>GSCKLPVKKATVVYQGERVKIQEKFKNGMLHGDKVSFFCKNKEKKCSYTEDAQCIDGTIEVPKCFKEHSS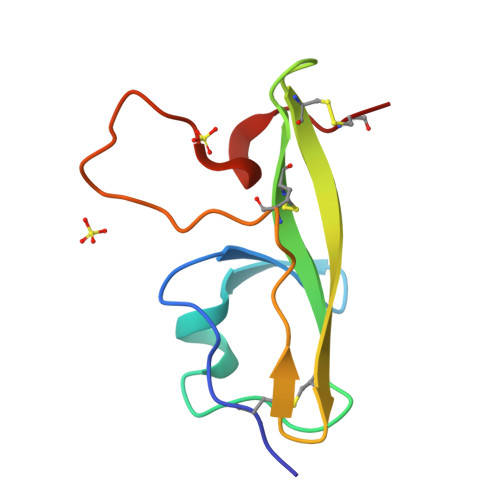LAFWKTDASDVKPCA[2x]>MQPFDSGHDDLVHDVVYDFYGRHVATCSSDQHIKVFKLDKDTSNWELSDSWRAHDSSIVAIDWASPEYGRIIASASYDKTVKLWEEDPDQEECSGRRWNKLCTLNDSKGSLYSVKFAPAHLGLKLACLGNDGILRLYDALEPSDLRSWTLTSEMKVLSIPPANHLQSDFCLSWCPSRFSPEKLAVSALEQAIIYQRGKDGKLHVAAKLPGHKSLIRSISWAPSIGRWYQLIATGCKDGRIRIFKITEKLSPLASEESLTNSNMFDNSADVDMDAQGRSDSNTEEKAELQSNLQVELLSEHDDHNGEVWSVSWNLTGTILSSAGDDGKVRLWKATYSNEFKCMSVITAQQ[2x];>MTIDDSNRLLMDVDQFDFLDDGTAQLSNNKTDEEEQLYKRDPVSGAILVPMTVNDQPIEKNGDKMPLKFKLGPLSYQNMAFITAKDKYKLYPVRIPRLDTSKEFSAYVSGLFEIYRDLGDDRVFNVPTIGVVNSNFAKEHNATVNLAMEAILNELEVFIGRVKDQDGRVNRFYELEESLTVLNCLRTMYFILDGQDVEENRSEFIESLLNWINRSDGEPDEEYIEQVFSVKDSTAGKKVFETQYFWKLLNQLVLRGLLSQAIGCIERSDLLPYLSDTCAVSFDAVSDSIELLKQYPKDSSSTFREWKNLVLKLSQAFGSSATDISGELRDYIEDFLLVIGGNQRKILQYSRTWYESFCGFLLYYIPSLELSAEYLQMSLEANVVDITNDWEQPCVDIISGKIHSILPVMESLDSCTAAFTAMICEAKGLIENIFEGEKNSDDYSNEDNEMLEDLFSYRNGMASYMLNSFAFELCSLGDKELWPVAIGLIALSATGTRSAKKMVIAELLPHYPFVTNDDIEWMLSICVEWRLPEIAKEIYTTL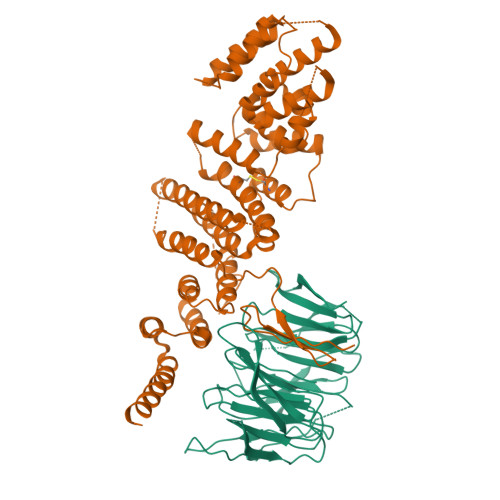GNQMLSAHNIIESIANFSRAGK[2x]> GHHHHHHEAIAKRLDACQDQLLELYEENSIDIHKHIMHWKCIRLESVLLHKAKQMGLSHIGLQ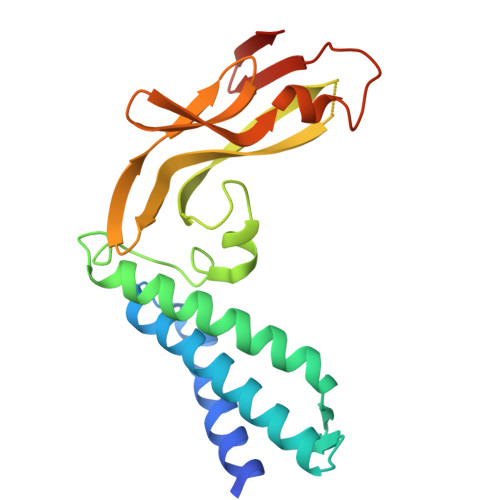VVPPLTVSETKGHNAIEMQMHLESLAKTQYGVEPWTLQDTSYEMWLTPPKRCFKKQGNTVEVKFDGCEDNVMEYVVWTHIYLQDNDSWVKVTSSVDAKGIYYTCGQFKTYYVNFNKEAQKYGSTNHWEVCYGSTVICSPASVSS>GPPGPPGGIRIEEIRDTAVALTWSRGTDNHSPISKYTIQSKTFLSEEWKDAKTEPSDIEGNMESARVIDLIPWMEYEFRIIATNTLGTGEPSMPSQRIRTEGAPPNVAPSDVGGGGGSNRELTITWMPLSREYHYGNNFGYIVAFKPFGEKEWRRVTVTNPEIGRYVHKDESMPPSTQYQVKVKAFNSKGDGPFSLTAVIYSAQDAPTEVPTDVSVKVLSSSEISVSWHHVTEKSVEGYQIRYWAAHDKEAAAQRVQVSNQEYSTKLENLKPNTRYHIDVSAFNSAGYGPPSRTIDI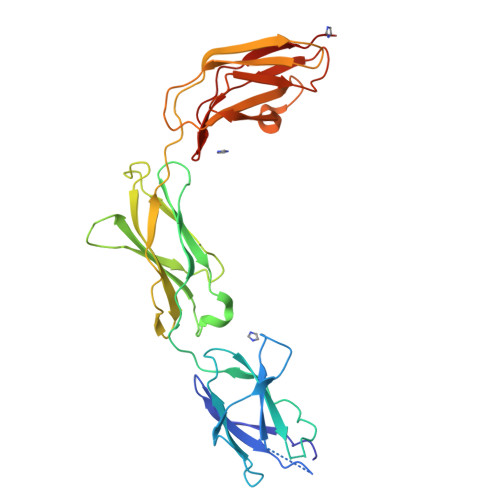ITRK[4x]>GHMATAPRPLREQYLHFQPISTRWHDNDIYGHVNNVTYYAFFDTAVNTYLIERGGLDIQGGEVIGLVVSSSCDYFAPVAFPQRIEMGLRVARLGNSSVQYELALFLEGQREACAAGRFVHVFVERRSSRPVA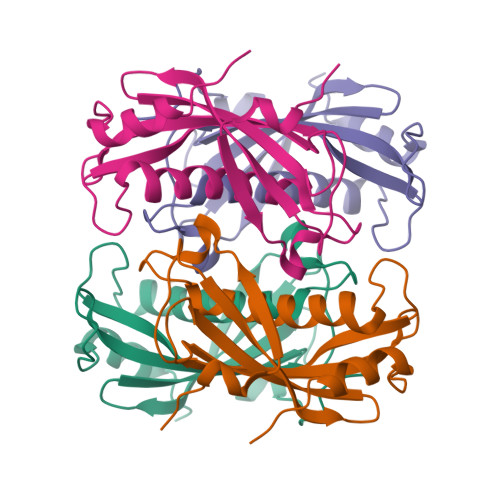IPQELRDALAALQSSAQ[6x]(1S)-1-(2,4-dichlorophenyl)-2-(1H-imidazol-1-yl)ethyl 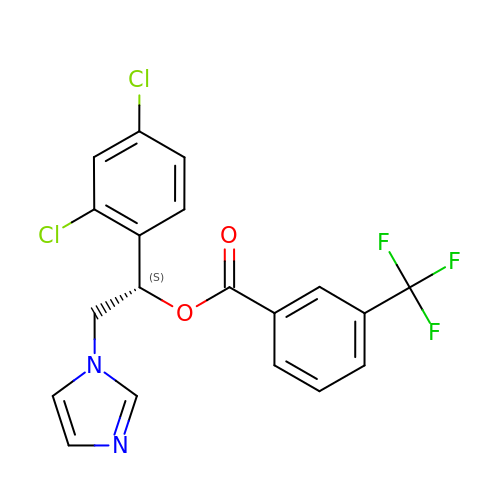3-(trifluoromethyl)benzoate | C19 H13 Cl2 F3 N2 O2 | SBOYKSSFXZSLMV-QGZVFWFLSA-N>[2x]GSSHHHHHHSQDPNSSSARLQQRAMGKTADRSLMASGHWVKIRVDASGVYRLTDEQLRANGFSDPSKVGVFGYGGGVLPEDLSRITTDDLPPVPVLRQGNALYFYAVGPVTWFYNPAKTTMEHTVNTYSTHGYYFLSDAAGAPLQMSQYTGGGASAEALIDYYDELMLHEQELYSPKESGRDLYGESFSAVNTRTVKFPLRGNTRSSGELGTVFSYIAKARSAGGGREMSLSANGILIFSDPFSMTSNEVSNSYLAGKKRRLYRSTPMNSLVNELRLDANYSMTGDAVNLDFIEVATQNDLRYDGAPMHIRRFSNLPVLGGESCRFVISEVPESLVVLQANSSLTASLVPVKTVGDKTIEFVAPPKGQDRRTINTFYAVDLSQASAPEILGAVPNQNLHGEEIPD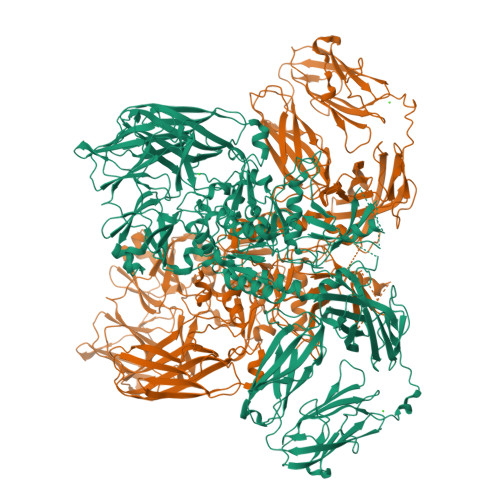LIIVSTQALLPEADRLATYRREKNGLKVLVVLQEQVFNEFSGGTPDATAYRLFAKMFYDRWKANAPVGETFPMQMLLFGDGAHDNRKVSVAWQKPYLQQTEFLLTFQAVNSTNVNSYVTDDYFGLLDDQPASVNIGWRNYNMAVGRFPVRTPAEARIAVDKTIRYEEDRESGAWRIRACFAADNGDKHATETSRLIDTVKRYAPAIMPVRAFQDVYPHVIENGLHSIPGAKKKMLETLQSGIILLNYAGHGGPAGWSDEHLLTLNDIHNFNYKHMPIWITATCDFANYDSQTTSAGEEVFLHEKSGTPIMFSTTRVVYNTQNEKINGFMLRRMFEKAKDGRYRTMGEIIRSAKQGMLSTVFPDSINQLSFFLMGDPSVRMNLPTHKVQLTAINGQDPEGQYGTIMLKSLERVALKGKVTDEKGTFDETFSGKVFLTVFDGRKKMTALEEEGNDLSLVYYDYPNVMYAGIAEVKDGLFETSFIVPKDVNYSEHEGRINLYAYNESTKAEAMGVDFSIRVQPGIPDEVTEDNTPPEIISCFLNDSTFRSGDEVNPTPLFMAEVFDLNGINITGSGVGHDITLCIDGRADLTYNLNAYFTSSATDAGVGTILFMIPALAEGDHTARLTVWDIFNNAVHHDFSFRVVDGIAPDVADVILFPNPVRESATFRIFHNRPGSDLNVVVEIYDFTGRLVNSLPVKTYSSSYGEPIEIKWDLTSKYGVKIGNGFYLYRCVVNSPGGQTASMAKKMIVVAQ> ADNTDGLAGFPRYKVANIQQVQQQIKSSGCAVYFFAYPLTDEPCFLVDLQALTGQQITEIPNPYYGKYAGPLGQIQTIKGVGPNGTIFAFSDV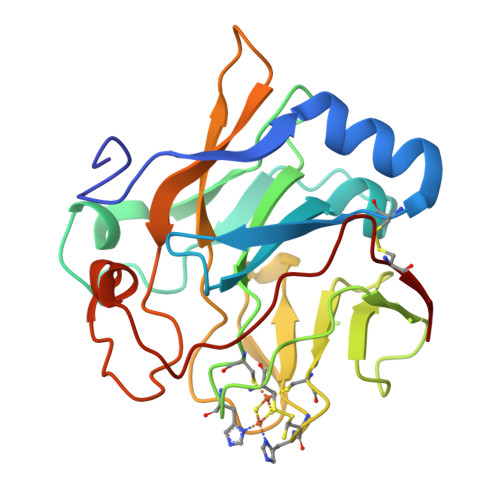CVHLGCQLPAQVIVSSESDPGLYAKGADLHCPCHGSIYALKDGGVVVSGPAPRPLPIVILDYDSSTGDIYAVGTNAPYFSAGIPRTTPQDNLLYDPRYSYSVPNNPSCSNG> GQNHHEVVKFMDVYQQSYCHPIETLVDIF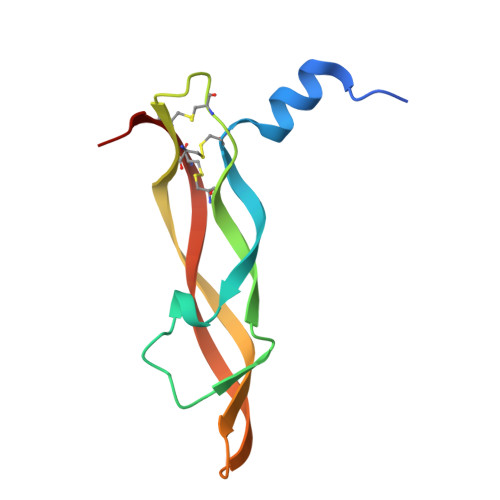QEYPDEIEYIFKPSCVPLMRCGGCCNDEGLECVPTEESNITMQIMRIKPHQGEHIGEMSFLQHNKCECRPKAD>[4x]GSRDPTQFEERHLKFLQQLGKGNFGSVEMCRYDPLQDNTGEVVAVKKLQHSTEEHLRDFEREIEILKSLQHDNIVKYKG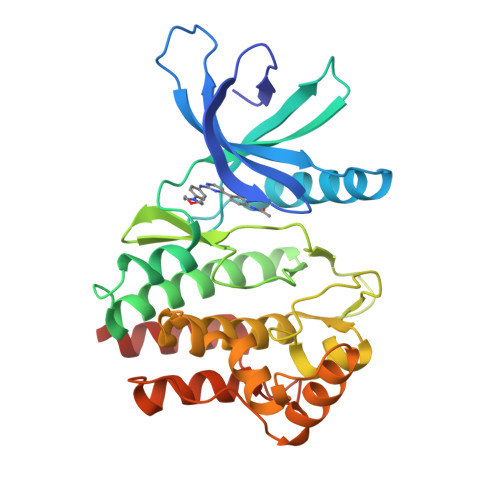VCYSAGRRNLKLIMEYLPYGSLRDYLQKHKERIDHIKLLQYTSQICKGMEYLGTKRYIHRNLATRNILVENENRVKIGDFGLTKVLPQDKEYYKVKEPGESPIFWYAPESLTESKFSVASDVWSFGVVLYELFTYIEKSKSPPAEFMRMIGNDKQGQMIVFHLIELLKNNGRLPRPDGCPDEIYMIMTECWNNNVNQRPSFRDLALRVDQIRDNMAGEF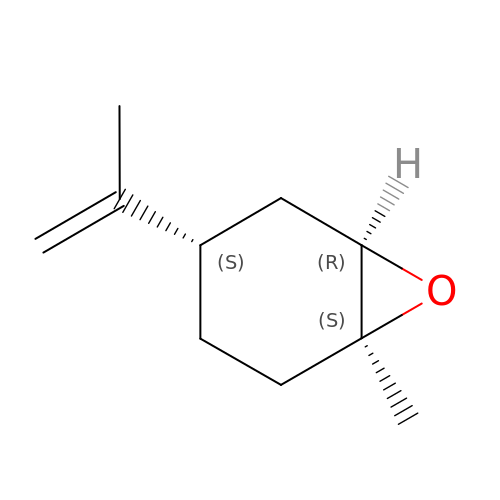(1S,4S,6R)-1-methyl-4-(prop-1-en-2-yl)-7-oxabicyclo[4.1.0]heptane | C10 H16 O | CCEFMUBVSUDRLG-AEJSXWLSSA-N> GPGSGLDSSHVGVRPSPATSQPTTSTGSADLDSILGHMGLPLGNSVLVEEQSTTEFHSILGKLFAAQGIVHNRISDSSADKTRNGDTHVIVLSLNQMFAKELPGIYKGSRKQMKKNLISEEESKVTVQNLNETQRSTPSRYKDLKIAWKYKLADEKRLGSPDRDDIQQNSEYKDYNHQFDITTRLMPAPIASELTFIAPTQPVSTILSQIEQTIKRNDKKLIRIVIPSLLHP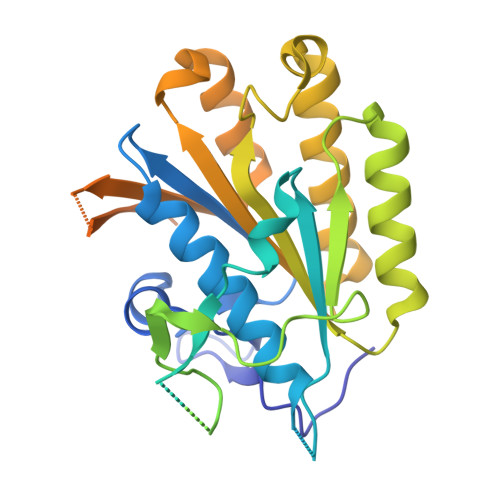AMYPPKMFESSEIIGLMHGVRSLVKKYYERVVLFASISIDIITPPLLVLLRNMFDSVINLEPFNQEMTEFLERVYKSQPGKIQHGLVHILKLPVFTDRGEMRVLKSEWAFKNGRKKFEIEQWGIPVDDAEGSAASEQSHSHSHS> MVEHDKSGSKRQELRSNMRNLITLNKGKFKPTASTAEGDEDDLSFTLLDSVFDTLSDSITCVLGSTDIGAIEVQQFMKDGSRNVLASFNIQTFDDKLLSFVHFADINQLVFVFEQGDIITATYDPVSLDPAETLIEIMGTIDNGIAAAQWSYDEETLAMVTKDRNVVVLSKLFEPISEYHLEVDDLKISKHVTVGWGKKETQFRGKGARAMEREALASLKASGLVGNQLRDPTMPYMVDTGDVTALDSHEITISWRGDCDYFAVSSVEEVPDEDDETKSIKRRAFRVFSREGQLDSASEPVTGMEHQLSWKPQGSLIASIQRKTDLGEEDSVDVIFFERNGLRHGEFDTRLPLDEKVESVCWNSNSEALAVVLANRIQLWTSKNYHWYLKQELYASDISYVKWHPEKDFTLMFSDAGFINIVDFAYKMAQGPTLEPFDNGTSLVVDGRTVNITPLALANVPPPMYYRDFETPGNVLDVACSFSNEIYAAINKDVLIFAAVPSIEEMKKGKHPSIVCEFPKSEFTSEVDSLRQVAFINDSIVGVLLDTDNLSRIALLDIQDITQPTLITIVEVYDKIVLLRSDFDYNHLVYETRDGTVCQLDAEGQLMEITKFPQLVRDFRVKRVHNTSAEDDDNWSAESSELVAFGITNNGKLFANQVLLASAVTSLEITDSFLLFTTAQHNLQFVHLNSTDFKPLPLVEEGVEDERVRAIERGSILVSVIPSKSSVVLQATRGNLETIYPRIMVLAEVRKNIMAKRYKEAFIVCRTHRINLDILHDYAPELFIENLEVFINQIGRVDYLNLFISCLSEDDVTKTKYKETLYSGISKSFGMEPAPLTEMQIYMKKKMFDPKTSKVNKICDAVLNVLLSNPEYKKKYLQTIITAYASQNPQNLSAALKLISELENSEEKDSCVTYLCFLQDVNVVYKSALSLYDVSLALLVAQKSQMDPREYLPFLQELQDNEPLRRKFLIDDYLGNYEKALEHLSEIDKDGNVSEEVIDYVESHDLYKHGLALYRYDSEKQNVIYNIYAKHLSSNQMYTDAAVAYEMLGKLKEAMGAYQSAKRWREAMSIAVQKFPEEVESVAEELISSLTFEHRYVDAADIQLEYLDNVKEAVALYCKAYRYDIASLVAIKAKKDELLEEVVDPGLGEGFGIIAELLADCKGQINSQLRRLRELRAKKEENPYAFYGQETEQADDVSVAPSETSTQESFFTRYTGKTGGTAKTGASRRTAKNKRREERKRARGKKGTIYEEEYLVQSVGRLIERLNQTKPDAVRVVEGLCRRNMREQAHQIQKNFVEVLDLLKANVKEIYSISEKDRERVNENGEVYYIPEIPVPEIHD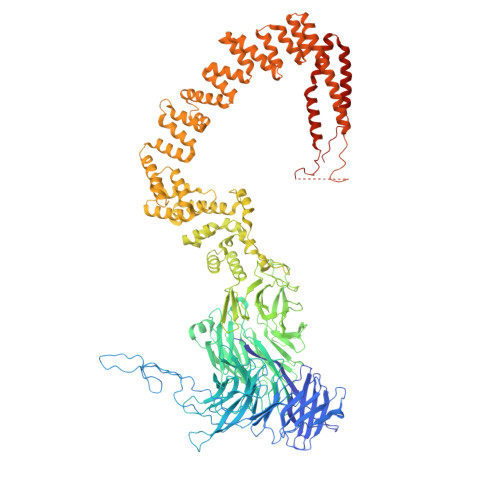FPKSHIVDF> GSMEISIDALMAKIKSTMMTREQIQKEYDALVKSSEDLLSALQKKKQQEEEAERLRRIQEEMEKERKRR

Myosin VI (Myo6) is the only minus-end directed nanomotor on actin, allowing it to uniquely contribute to numerous cellular functions. As for other nanomotors, the proper functioning of Myo6 relies on precise spatiotemporal control of motor activity via a poorly defined off-state and interactions with partners. Indeed, while they are back-folded monomers in their inactive form, these motors can self-associate to form active dimers upon activation. TOM1 and Dab2 cannot bind the off-state, while GIPC1 binds Myo6, releases its auto-inhibition and triggers proximal dimerization.

SEC-MALS with six fragments derived from the 3HB/SAH junction indicated that a rather conserved region (aa 875–940) can self-dimerize with KDApp of ~19 µM (∆G° ~−6.4 kcal/mol) obtained from titration. This minimal region corresponds to the last half of the 3HB (i.e., the 2nd and 3rd helix) and the first part of the SAH. Crystals of the 875–940 peptide diffracted to 2.1 Å resolution. Clear electron density for all residues from 876 to 937 indicates that they form an extended helix that dimerizes in an antiparallel manner. This antiparallel dimerization is stabilized by multiple apolar contacts involving 13 residues from each helix, and six polar interactions involving R892 with D900, and T888 with S906 (via a water molecule). At the center of the interface, the structure highlights how residues T888, R892 and V903 contribute to the dimerization. Three mutations (T888D.R892E.V903D) were introduced into the 875–940 peptide to assess the impact on proximal dimerization. SEC-MALS confirms that the T888D.R892E.V903D mutant stays monomeric even up to 43 µM (peak concentration in the SEC-MALS experiment) while the WT counterpart is dimeric in similar conditions. The inter-head distance is indeed compatible with the large (~30 nm) stepping previously reported when Myo6 walks processively. Myo6 is unique in that its antiparallel coiled-coil and Lever arm in the dimer are derived from the unfolding of a 3HB, with the contribution of the SAH.>[4x]SNAMSEDNYRTIALAFLDESADSTTINA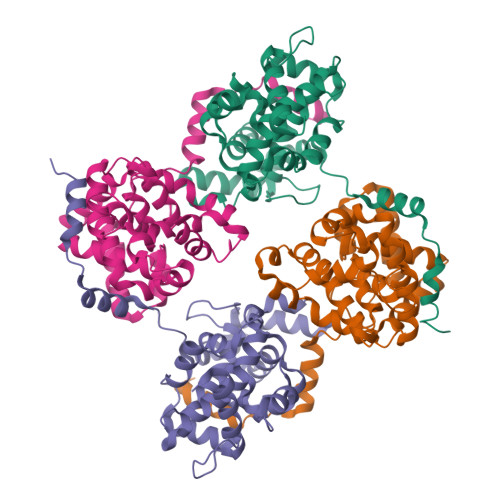WVNEFAYQGFDPKRIVQLVKERGTAKGRDWKKDVKMMIVLNLVDGNEPESMMKEMSEKGAAIVTQLISTYQLKEGNPGRDTITLSRVSAAFVPWTVQALKTLSESLPVTGTTMDSIAGTTYPRCMMHPSFAGIIDLELPNNTGAMLADAHGLFMLEFSKTINPSLRTKQPNEIAATFEKPNMAAMTGRFFTRDDKKKLLIAIGVLNEDLVPNPAIEKCAEKYKAKVGKV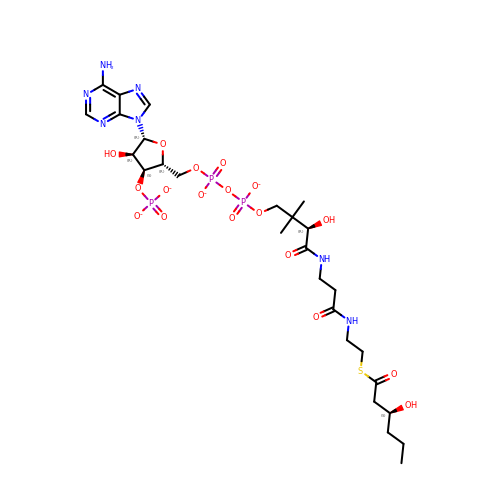(S)-3-Hydroxyhexanoyl-CoA | C27 H42 N7 O18 P3 S | VAAHKRMGOFIORX-IKTBLOROSA-J> MTSLIDLGRYVERTHHGEDTEPRSKRVKIAKPDLSSFQPGSIIKIRLQDFVTYTLTEFNLSPSLNMIIGPNGSGKSTFVCAVCLGLAGKPEYIGRSKKVEDFIKNGQDVSKIEITLKNSPNVTDIEYIDARDETIKITRIITRSKRRSDYLINDYQVSESVVKTLVAQLNIQLDNLCQFLSQERVEEFARLKSVKLLVETIRSIDASLLDVLDELRELQGNEQSLQKDLDFKKAKIVHLRQESDKLRKSVESLRDFQNKKGEIELHSQLLPYVKVKDHKEKLNIYKEEYERAKANLRAILKDKKPFANTKKTLENQVEELTEKCSLK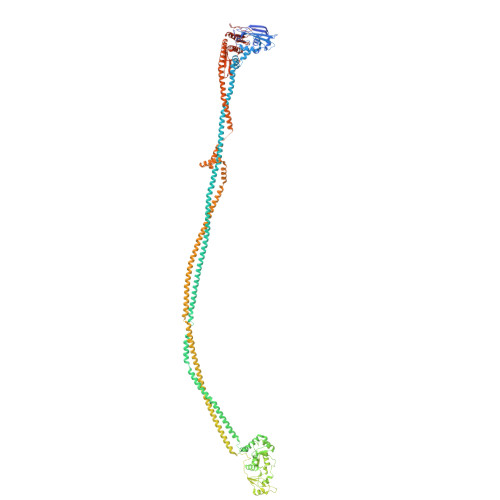TDEFLKAKEKINEIFEKLNTIRDEVIKKKNQNEYYRGRTKKLQATIISTKEDFLRSQEILAQTHLPEKSVFEDIDIKRKEIINKEGEIRDLISEIDAKANAINHEMRSIQRQAESKTKSLTTTDKIGILNQDQDLKEVRDAVLMVREHPEMKDKILEPPIMTVSAINAQFAAYLAQCVDYNTSKALTVVDSDSYKLFANPILDKFKVNLRELSSADTTPPVPAETVRDLGFEGYLSDFITGDKRVMKMLCQTSKIHTIPVSRRELTPAQIKKLITPRPNGKILFKRIIHGNRLVDIKQSAYGSKQVFPTDVSIKQTNFYQGSIMSNEQKIRIENEIINLKNEYNDRKSTLDALSNQKSGYRHELSELASKNDDINREAHQLNEIRKKYTMRKSTIETLREKLDQLKREARKDVSQKIKDIDDQIQQLLLKQRHLLSKMASSMKSLKNCQKELISTQILQFEAQNMDVSMNDVIGFFNEREADLKSQYEDKKKFVKEMRDTPEFQSWMREIRSYDQDTKEKLNKVAEKYEEEGNFNLSFVQDVLDKLESEIAMVNHDESAVTILDQVTAELRELEHTVPQQSKDLETIKAKLKEDHAVLEPKLDDIVSKISARFARLFNNVGSAGAVRLEKPKDYAEWKIEIMVKFRDNAPLKKLDSHTQSGGERAVSTVLYMIALQEFTSAPFRVVDQINQGMDSRNERIVHKAMVENACAENTSQYFLITPKLLTGLHYHEKMRIHCVMAGSWIPNPSEDPKMIHFGETSNYSFD SPH1118 has been identified as a pectin-binding protein involved in both pectin chemotaxis and assimilation. SPH1118 shows high homology with the solute-binding protein (SBP) associated with the bacterial ABC transporter. SPH1118 consisted of two domains with a large cleft between the domains and substrates bound to positively charged and aromatic residues in the cleft through hydrogen bond and stacking interactions. Here we show tertiary structures of SPH1118 with six different conformations as determined by X-ray crystallography.

Interestingly, SPH1118 showed three conformations [SPH1118 (open form), SPH1118 (full open form), and SPH1118 (closed form)] even in the substrate-free state. The crystallization conditions of SPH1118 (open form), SPH1118 (full open form), and SPH1118 (closed form) contained the substrates (ΔtriGalUA or sodium PG). However, no substrates were bound to SPH1118 in these structures. The crystal structures of SPH1118 (full open form) and SPH1118 (closed form) were obtained only under crystallization conditions in the presence of sodium PG. Two molecules were included in the asymmetric unit of the crystals of SPH1118 (closed form) and SPH1118/ΔtriGalUA. Root mean square deviations (RMSDs) between two monomers in the same crystals were calculated, respectively, indicating that there were few structural differences [SPH1118 (closed form), 0.543 Å; SPH1118/ΔtriGalUA, 0.106 Å]. Compared to the C terminal domain of SPH1118 (full open form), those of SPH1118 (open form) and SPH1118 (closed form) were closed by 18.9° and 34.2°, respectively, suggesting that the domain of SPH1118 was flexibly opened and closed even in the substrate-free state. There are a few examples of proteins whose domains are closed in the substrate-free state, as observed in SPH1118 (closed form). There is little structural difference between the closed forms in the substrate-free state and the substrate-bound state. Further studies are necessary to elucidate the physiological significance of SBPs adopting the closed conformation in the absence of the substrate.

>[2x]AAFTQAPMLEQNKQLPPVDQRLPEKPLVIKPIASNGVYGGTLRTVMRGNADGNGILRTIGPQGLTHWTQDIQTVEPYVAESYTVSPDAMEYTFKLRKGMKWSDGTPFTADDIVFAMNDVVLNKEMFPQTPSAYLVGGKAPKVSKVDDYTVKFEFPAANLSFPETLATPLGQHPTLYQKKYCSQFHPAYNKNVQAEFTKANVKDWPSLMRAKCSDIELPSRWSSTERPSIDPWLIKEPYGGAVTRVVMERNPFYWQVDPTGKQLPYVDRIQYAVVSDLQAIILAATNGQYDIEARLLGSDVTSRPLMLKNQQKGGYKVFGQTSANANAAGLWLNQTTKNEKLRKYMTQHDFRQALSLAMDRDEINKVAWLGQAAPWQSGPFKESKWYNEKLATQYLKLDLAQANQILDRLGLTKRDSDGYRTYPDGGRVSLDAIVMIDRQAMVQTLELIRRQWQKAGVELVIKGSERSLFYNRATANDYDISIDVFPGGLDATLNPRAYVAVHPLESRMSLEWAKWYLSGGKQGIEPNESMKKRMALYDQFVAAKTQSQALSLFKQILQISADEFEVIGTVRPAVISSLHSLKLQNVNEKMPFGWPYATPSLSLPQQWYFSKLEHHHHHH In this work, we exhaustively probe the ability of all 36 immobile HJ sequences to form DNA crystals in two different designed systems. Three separate self-assembling DNA crystal systems are described in this report: the “4 × 5” and “4 × 6” designs (collectively referred to as the 4 × N systems), and a third construct with a “scrambled” sequence variant of the 4 × 6 lattices. Self-assembly was mediated by three constituent oligonucleotides: (S1) containing four sequence repeats of either 5 or 6 bases; (S2) composed of 21 bases containing complementary regions to both (S1); and (S3) which forms the second junction crossover. The HJ serves as the fundamental component at the core of each unit, and the ultimate assembly of the full lattice is facilitated by the complementary 2-base sticky ends that tail each duplex.

The 4 × 5 system robustly crystallized with 75% of the junctions, and we obtained crystals in all but 9 of 36 sequences. Of the resulting structures, 18 exhibited P32 symmetry with average cell dimensions a = b = 68.85 Å c = 60.09 Å, with only nine retaining the original P3221 symmetry with average cell edges a = b = 68.17 Å c = 60.60 Å. Although the cell parameters between the two symmetries were virtually indistinguishable, the differences between the periodicity of the lattices is dramatic, with vastly different cavity sizes. Pos1 and 2 were readily observable in the electron density maps at either one or both of these conserved sites in a significant number of the structures, with no apparent respect to motif or symmetry. However, in the majority of the crystal structures reported here, the cacodylate anion indeed fits best into the electron density map of our X-ray structures, due to the presence of sodium cacodylate in the crystallization solution.

> GAGCAGACCAG;> ACGCCACTCA;> CTCGT;> TCTGAGTGGGGTCTGC>DLPLTHTALFKQVPLDQARELLEHLHESVFSKGQAIFNEGDTDRRMYLLERGRVKLVRHSRDNRVQLLSIHTHGEILGEIPVFDPFGGPRTASAIAITDRTRVLWLENEVLFKWLGHHPRVAVDMLQVLAARLRANNEHISDLVFMDVPARLAKTLLNLASRFGEPVREGVLVPHDLTQEELAQLVGSSRETVNKALMDFAQR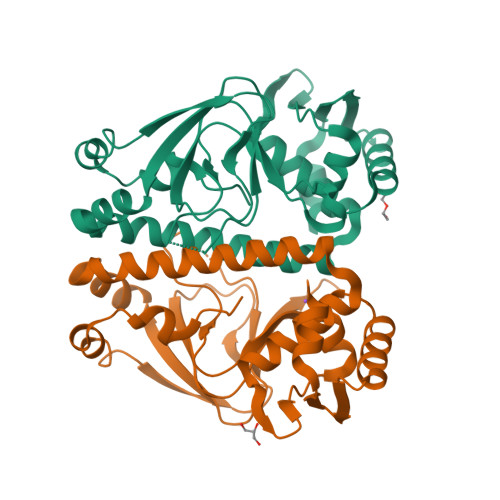GWIKRHGRSIIIYQPGMLIRRAE[2x]> MFSTNTVLWARALVDRKSPQLWGAPGAPIIRMR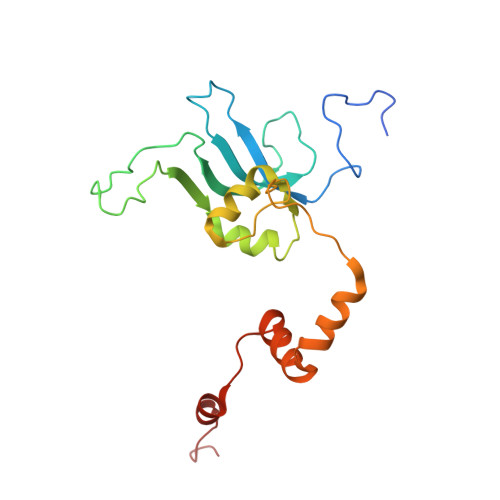GHHVTWKFQSYDMFVEHTHRRRNSDIRLLHYLGKHCPHPQKSLWSPDTPVTQDRHLFMLTTIDVDAFKYWFGVKRCRLSVGPWNILAKSGLLPPSYKQNSKIMPKPIFDKEQLMRYYLANRKDQRQMEREDYLNYKNSMVKSPEERAAERPVAPFL>MKAVQYTEIGSEPVVVDIPTPTPGPGEILLKVTAAGLCHSDIHVMDMPAAQYALGLPLTLGHEGVGTVAELGEGVT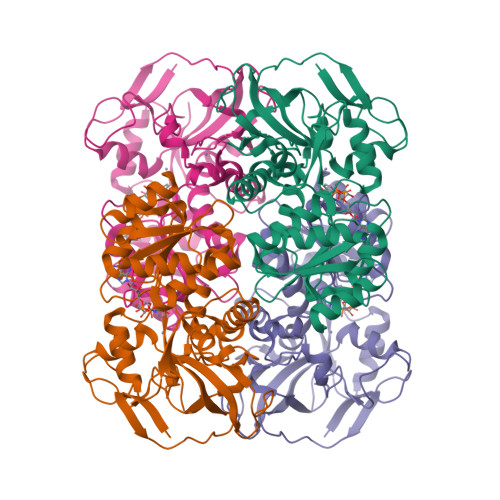GFGVGDAVAVYGPWGCGACHACARGRENYCTRAADLGITPPGLGSPGSMAEYMIVDSARHLVPIGDLDPVAAAPLTDAGLTPYHAISRVLPLLGPGSTAVVIGVGGLGHVGIQILRAVSAARVIAVDLDDDRLALAREVGADAAVKSGAGAADAIRELTGGQGATAVFDFVGAQSTIDTAQQVVAVDGHISVVGIHAGAHAKVGFFMIPFGASVVTPYWGTRSELMEVVALARAGRLDIHTETFTLDEGPAAYRRLREGSIRGRGVVVPTSHHHHH[4x]>MALRTMVDPDTCTSCELCYDRVPEVYKNRGDGIAEVVSPGPDGWMMVPPELEQEVKEVTDECPAGSIITEE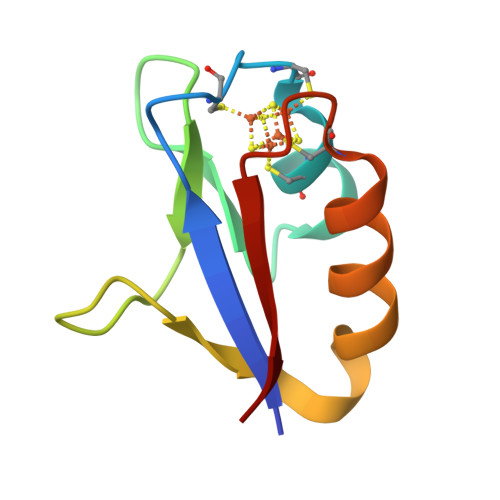V[2x]>[2x]SAEIQPRSDEKRILSNVAVLEGAPPLSEHWQLFNNNEVLFNEARTAQAATVVFSLQQNAQIEPLARSIHTLRRQRGSAMKILVRENTASLRATDERLLLACGANMVIPWNAPLSRCLTMIESVQGQKFSRYVPEDITTLLSMTQPLKLRGFQKWDVFCNAVNNMMNNPLLPAHGKGVLVALRPVPGIRVEQALTLCRPNRTGDIMTIGGNRLVLFLSFCRINDLDTALNHIFPLPTGDIFSNRMVWFEDDQISAELVQMRLLAPEQWGMPLPLTQSSKPVINAEHDGRHWRRIPEPMRLLDDAVERSS

Bacterial cellulose is a widespread biofilm component whose secretion in Gram-negative species requires an inner membrane, c-di-GMP-dependent synthase tandem (BcsAB), an outer membrane porin (BcsC), and various accessory subunits that regulate synthase assembly and function as well as the exopolysaccharide’s chemical composition and mechanical properties. A third cytosolic protein, BcsE, has been shown to significantly boost cellulose secretion in vivo and to present a second c-di-GMP binding module in addition to the BcsAPilZ domain. Crystallographic and solution-based data show that BcsE’s predicted GIL domain is a degenerate receiver-GGDEF domain tandem (BcsEREC*-GGDEF*), where the divergent diguanylate cyclase module binds both dimeric c-di-GMP and BcsQ through mutually independent interfaces. In addition, we reveal that a third N-terminal domain (BcsENTD) determines the protein’s homooligomerization and targeting of BcsERQ to the membrane as well as previously unreported interactions with transcription antitermination complex components. Together, the data suggest that BcsE acts on multiple levels to fine-tune bacterial cellulose secretion, from the early stages of secretion system assembly to the maintenance of a membrane-proximal pool of dimeric c-di-GMP for processive synthase activation.

Purified untagged BcsE217−523 crystallized in the presence of c-di-GMP, and its structure was determined to 2.2 Å using single-wavelength anomalous dispersion (SAD) phasing on crystals grown from selenomethionine-derivatized protein. The protein packed in the P41212 space group with two BcsE217−523 molecules per asymmetric unit adopting virtually identical conformations with root mean square deviation (RMSD) of 0.835 Å over all atoms. A single c-di-GMP is found splayed in a symmetrical conformation between the two protomers, and nucleotide recognition involves four residues of each subunit, namely, R415 and D418 from the conserved I site-like motif as well as the side chain of H445 and the peptide carbonyl of S432. Unexpectedly, the construct adopts a dual-domain fold with an apparent N-proximal module connecting via an interstitial helix (α6) to a C-terminal domain, in which the last ∼40 residues (C-terminal tail) remain unresolved in the structure. A search for three-dimensional (3D) structural homologs using the fold recognition server DALI revealed that the N-proximal domain adopts a receiver (REC) domain-like (βα)5 fold, where the central five-stranded parallel β-sheet is flanked by 4 α-helices, while the canonical α1 is mostly unfolded in an extended conformation by a stretch of proline and other small uncharged amino acids. Structural and sequence alignments of BcsEREC* with phosphorylation-competent receiver domains, however, show significant deviation from the amino acid consensus of key functional motifs, indicating that the module is unlikely to function in phosphotransfer-dependent signal transduction.> CDY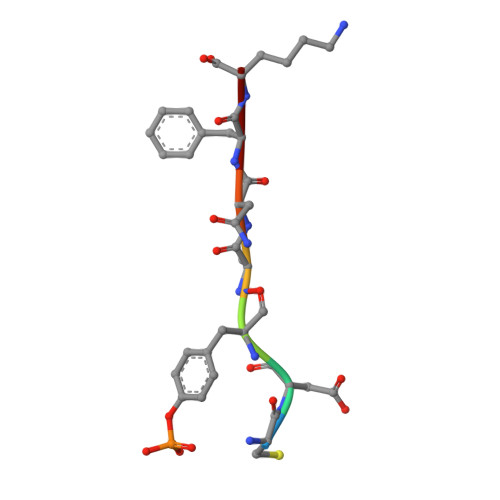ANFK>HMSIITDVYAREVLDSRGNPTLEVEVYTESGAFGRGMVPSGASTGEHEAVELRDGDKSRYLGLGTQKAVDNVNNIIAEAIIGYDVRDQQAIDRAMIALDGTPNKGKLGANAILGVSIAVARAAADYLEVPLYTYLGGFNTKVLPTPMMNIINGGSHSDAPIAFQEFMIMPVGAPTFKEGLRWGAEVFHALKKILKERGLVTAVGDEGGFAPKFEGTEDGVETILKAIEAAGYEAGENGIMIGFDCASSEFYDAERAVYDYTKFEGEGAAVRTSAEQVDYLEELVNKYPIITIEDGMDENDWDGWKVLTERLGKRVQLVGDDFFVTNTEYLARGIKENAANSILIKVNQIGTLTETFEAIEMAKEAGYTAVVSHRSGETEDSTIADIAVATNAGQIKTGSLSRTDRIAKY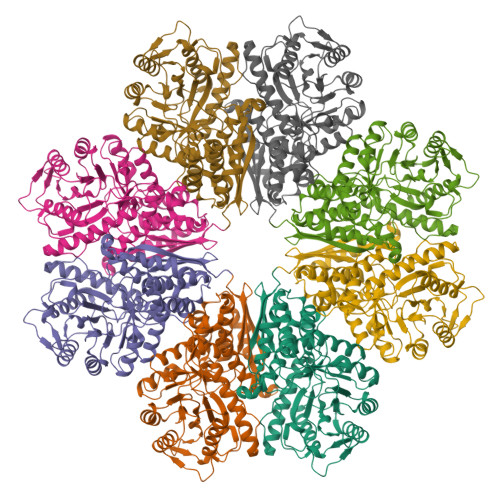NQLLRIEDQLGEVAQYKGIKSFYNLAA[8x]>MAGLYTTYQLLEVQRKLKTLPAFFLQWFPRQINFQEDMIAFDKVIQDVTRVAPFVAPNVQGRVIKESGYNTKTFKPAYVKPKHVIDPNMIIPRQPGEALGTGTLSIAQRRDRVIAYLLMKHRAMHENTWEWMAAQAAQYGYVDVQGQDYPLVRVDFGRDAALTMTTDWTAAGVTLMDMIADLRDGQRLVSDKSMSGTVIRDYVFGGDAWDQFVKVGGKELWGKDGLMDSTIRGSETNVTRLWDDVEGVQYMGELVGANGAGRMRIWVNTQKYRDQNDQEQFLMKQKAVMGISSAIEGVRCFGAILDKGAGYQALDYFPKMWDQEDPSVEYLMSQGAPLMVPADPNASFLLTVMS[7x];>MNLLTMMAATSLPNYLAGNGDLGSWEPTQIFAGEADIVTEGGAAGADIEIYQVIAKNAAGAMVPHDPTATTGTSPDEVPAPQSVAIGIAAQPAKSGQNVPYY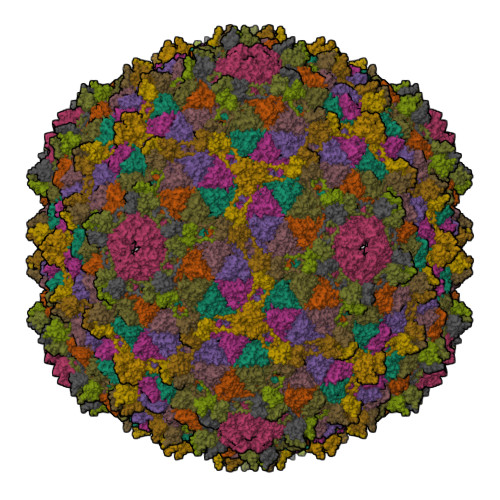IGGVFNHAALGWHASLDTLAKRQAVFDRTNIHIGNLY[7x]>MKDYKSITIATEGSYAPYNFKDAGGKLIGFDIDLGNDLCKRMNIECKFVEQAWDGIIPSLTAGRYDAIMAAMSIQPAREKVIAFSRPYLLTPMTFLTTADSPLLKTQVAIENLPLDNITPEQKAELDKFTKIFEGVKFGVQAGTSHEAFMKQMMPSVQISTYDTIDNVVMDLKAGRIDASLASVSFLKPLTDKPDNKDLKMFGPRMTG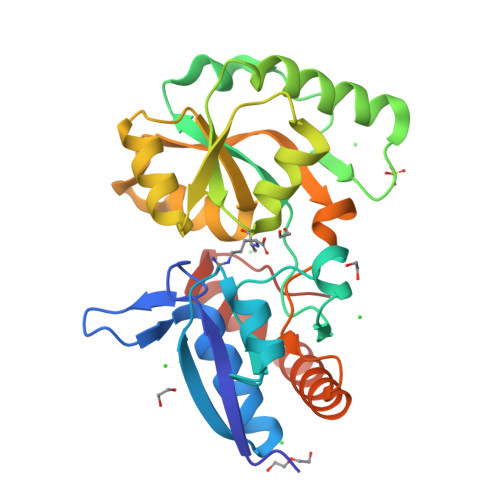GLFGKGVGVGIRKEDADLKALFDKAIDAAIADGTVQKLSQQWFGYDASPKQHHHHHH[2x]>[8x]GSHMATNDE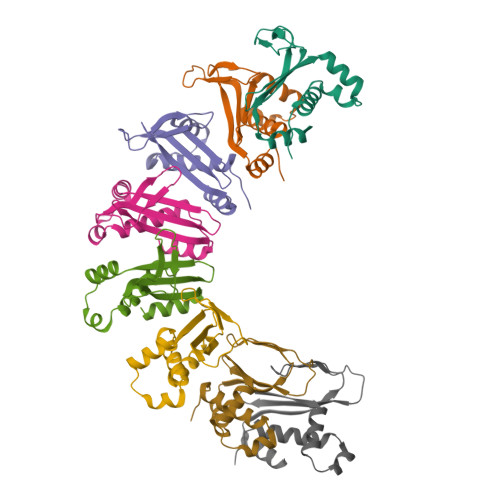LKNQLANKQNGGQVASAQSLDLKGLLEAPTMRKKFEKVLDKKAPQFLTSLLNLYNGDDYLQKTDPMTVVTSAMVAATLDLPIDKNLGYAWIVPYKGRAQFQLGYKGYIQLALRTGQYKSINVIEVREGELLKWNRLTEEIELDLDNNTSEKVVGYCGYFQLINGFEKTVYWTRKEIEAHKQKFSKSDFGWKKDYDAMAKKTVLRNMLSKWGILSIDMQTAVTEDEAEPRERKDVTDDESIPDIIDAPVTPSDTLEAGSVVQGSMI>MLVSVYLALLVACVGQAHSQANLMRLKSDLFNRSPMYPGPTKDDPLTVTLGFFLQDIVKVDSSTNEVDLVYYERQRWKLNSLMWDPNEYGNITDFRTSAADIWTPDITAASSTRPVQVLSPQIAVVTHDGSVMF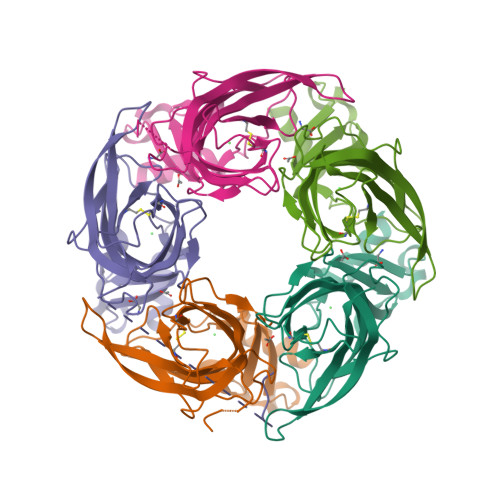SPAQRLSFMCDPTGVDSEEGVTCAVKFESWVYSGFEIDLKTDTDQVDLSSYYASSKYEILSATQTRQVQHYKGTGEPYIDVNLVVKFRERRAGNGFFRNLFDENLYFQGHHHHHH[5x]>[8x]MAEAASCARKGTKYAEGTQPFTVLIEGNIGSGKTTYLNH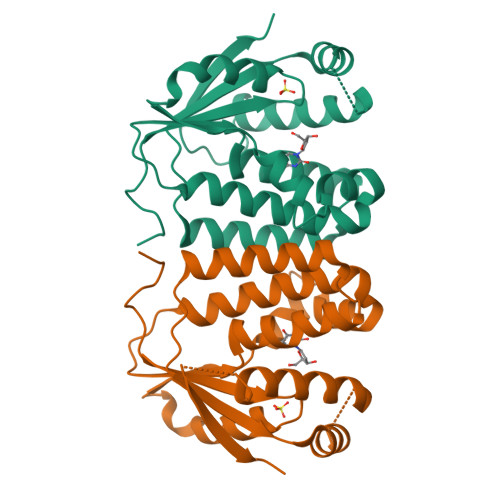FEKYKNDICLLTEPVEKWRNVNGVDLLELMYKDPKKWAMPFQSYVTLTMLQSHTAPTNKKLKIMERSIFSARYCFVENMRRNGSLEQGMYNTLEEWYKFIEESIHVQADLIIYLRTSPEVAYERIRQRARSEESCVPLKYLQELHELHEDWLIHQRRPQSCKVLVLDADLNLENIGTEYQRSESSIFDAIS>[2x]SNANKYNKIANELIKIIGEDNIISITHCATRLR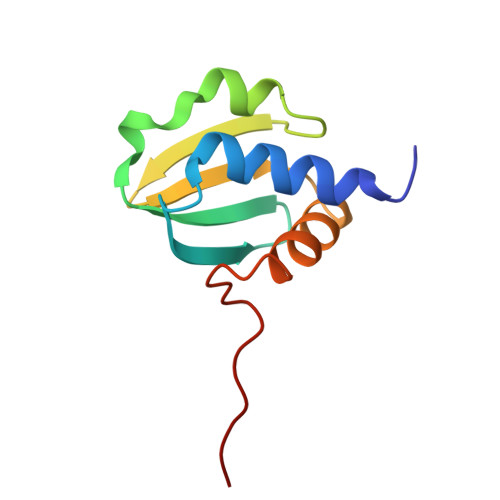VMVKDREIINDKKVEKVDEVKGVFFTSGQYQIILGTGIVNKVYAEVEKMGLKTLSKKEQDEL>[2x]AVPDAVDWREKGAVTPVKDQGACGSCWAFSAVGNIEGQWYLAGHELVSLSEQQLVSCDDMDNGCSGGLMLQAFDWLLQNTNGHLHTEDSYPYVSGNGYVPECSNS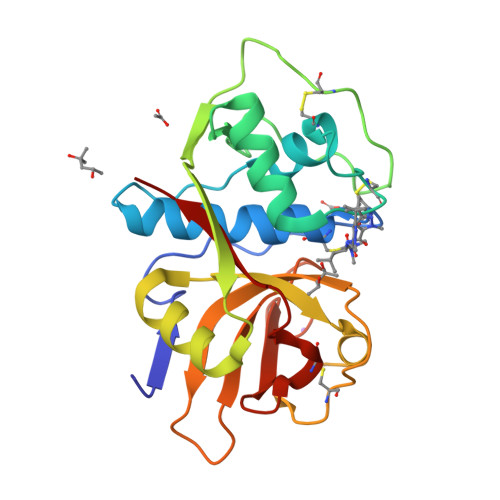SELVVGAQIDGHVLIGSSEKAMAAWLAKNGPIAIALDASSFMSYKSGVLTACIGKQLNHGVLLVGYDMTGEVPYWVIKNSWGGDWGEQGYVRVVMGVNACLLSEYPVSAHVR> GPKVPMSQKNGIATLLQAEKEAHEIVSKARKYRQDKLKQAKTDAAK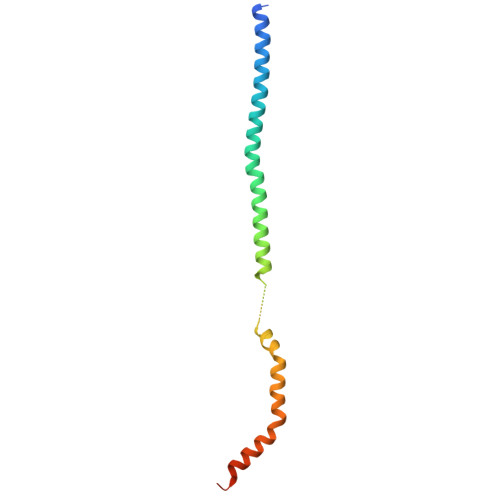EIDSYKIQKDKELKEFEQKNAGGVGELEKKAEAGVQGELAEIKKIAEKKKDDVVKILIETVIKPSAEVHINAL> AAPLAATASKFLGCAYGAQQAPGFAQYWNKLTPENGGKWGSVEAVRDQMDWSTLDAAYRFAQANQMPFQMHVM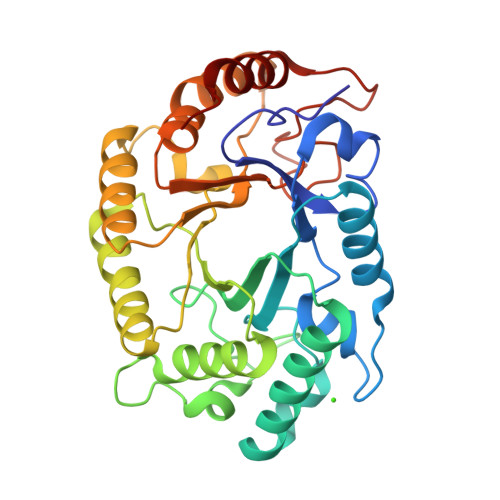VWGNQQPEWIKTLRPAEQRREIEQWFAAVAQRYPDIALLEVVNEPLNDPPSKADTGGGNYLQALGGNGDSGWEWVLQSFRLARRHFPHTKLMINDYSITSSAQATQKYLQIVRLLQRENLVDAIGVQEHAFETTPEVAVSVHRDNLDALAATGLPIYITEFDLDGPTDAQQLADYKRVFPVFWEHPAVHGITLWGFRPGLWRDKEAAYLIRADGTERPALTWLRDYVAAHPGT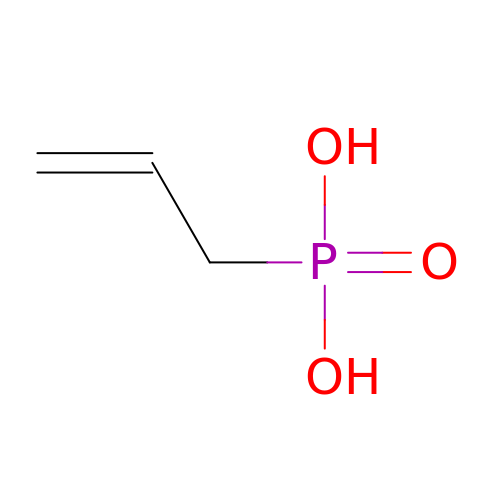prop-2-en-1-ylphosphonic acid | C3 H7 O3 P | RZKYDQNMAUSEDZ-UHFFFAOYSA-N> 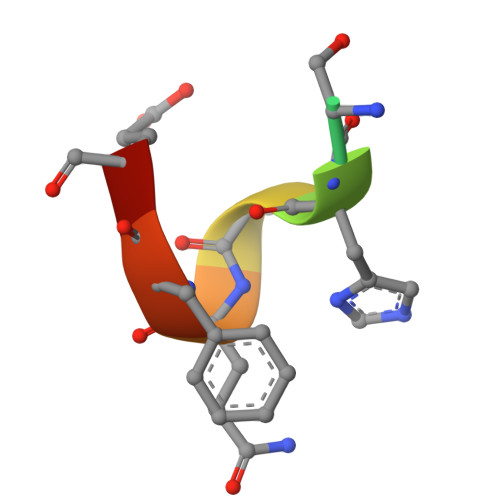NWSHPQFEK> MGDKLSKTDWKIVSFTTEEASGEGSNNGHAKHLIDGNIETFWHSRWQGGSDPLPYEIIIDMNHRVKIAQIELLPRGRGSNNPIKVVRFEASEDGTNWES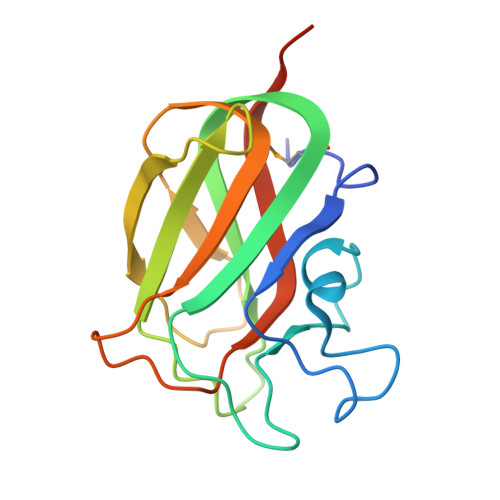IGQFGFTNQDAALKYYVKSSTARYIKLVIPDGVGNGTVAAIRELDVRGTVVNLEHHHHHH(E)-4-((tetrahydro-2H-pyran-2-yloxyimino)methyl)benzimidamide 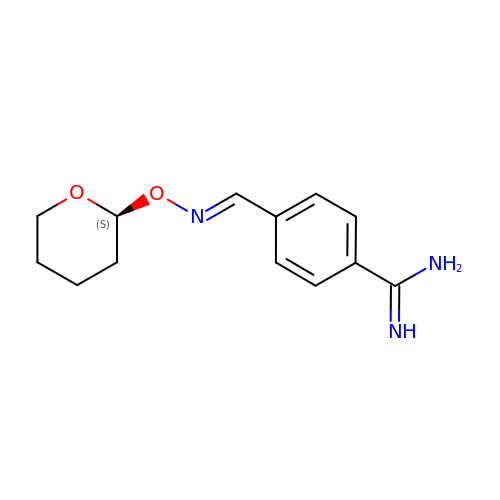| C13 H17 N3 O2 | WEPKQSGLGGDMSU-RGZVIEDOSA-N>MAHHHHHHVGTNTGGVLVITDTIIVKSGQTYDGKGIKIIAQGMGDGSQSQNQKPIFKLEKGANLKNVIIGAPGCDGIHCYGDNVVENVVWEDVGEDALTVKSEGVVEVIGGSAKEAADAVFQLNAPCTFKVKNFTATNIGKLVRQNGNTTFKVVIYLEDVTLNNVKSCVAKSDSPVS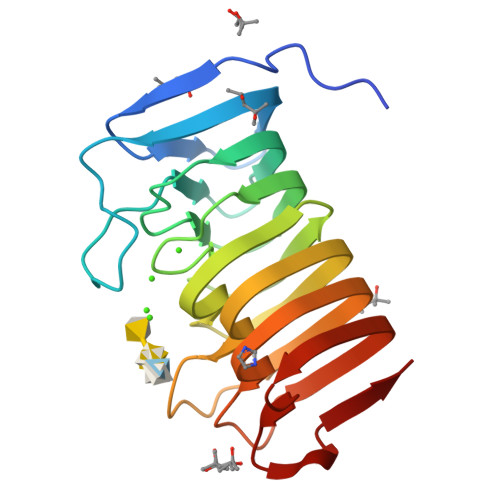ELWYHNLNVNNCKTLFEFPSQSQIHQY[2x]> AEIQWMRPSKEVGYPIINAPSKTKLEPSAFHYVFEGVKEPAVLTKNDPRLKTDFEEAIFSKYVGNKITEVDEYMKEAVDHYAGQLMSLDINTEQMCLEDAMYGTDGLEALDLSTSAGYPYVAMGKKKRDILNKQTRDTKEMQKLLDTY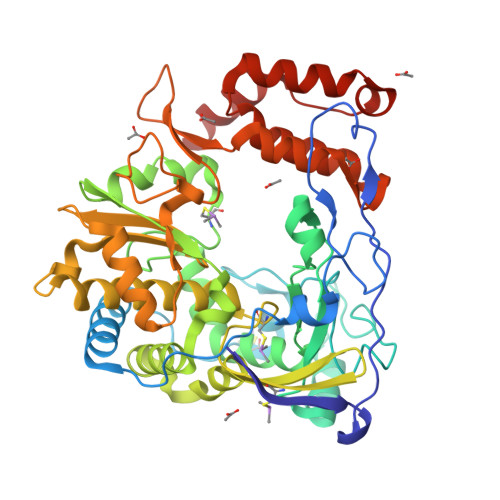GINLPLVTYVKDELRSKTKVEQGKSRLIEASSLNDSVAMRMAFGNLYAAFHKNPGVITGSAVGCDPDLFWSKIPVLMEEKLFAFDYTGYDASLSPAWFEALKMVLEKIGFGDRVDYIDYLNHSHHLYKNKTYCVKGGMPSGCSGTSIFNSMINNLIIRTLLLKTYKGIDLDHLKMIAYGDDVIASYPHEVDASLLAQSGKDYGLTMTPADKSATFETVTWENVTFLKRFFRADEKYPFLIHPVMPMKEIHESIRWTKDPRNTQDHVRSLCLLAWHNGEEEYNKFLAKIRSVPIGRALDLPEYSTLYDRWLDSF6-MORPHOLIN-4-YL-9H-PURINE | C9 H11 N5 O | 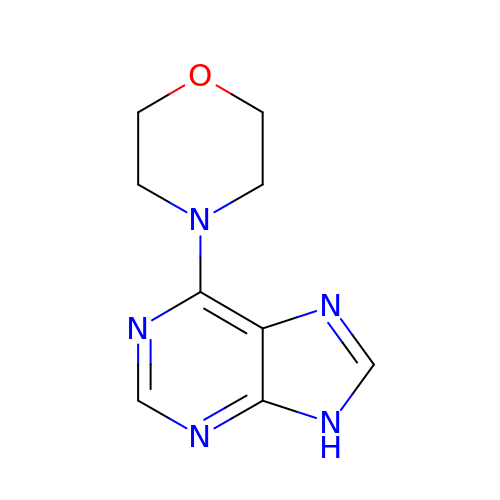MEOMXKNIFWDDGZ-UHFFFAOYSA-N EhCoactosin, an actin-binding protein of the ADF/cofilin family, participates in actin dynamics, and here we report our studies of this protein using both structural and functional approaches. According to in vitro binding assays, full-length EhCoactosin binds both F- and G-actin. Instead of acting to depolymerize or severe F-actin, EhCoactosin directly stabilizes the polymer. When EhCoactosin was visualized in E. histolytica cells using either confocal imaging or total internal reflectance microscopy, it was found to colocalize with F-actin at phagocytic cups.

EhCoactosin consists of a central core of β-sheets surrounded by α-helices. The central core is made up of five strands: β1(26–32), β2(37–44), β3(60–69), and β4(76–85) forming antiparallel strands while β5-strand (113–117) forms parallel strand with β3 and β4. The central β-sheets are flanked on both sides by a total of five helices; α1(9–17) and α3(92–107) are located on the N-terminal side, and α2(48–54), α4(120–122) and α5(125–137) are located on the C-terminal side. This arrangement of secondary structural elements is a common structural feature of proteins belonging to the ADF/cofilin family. The loop connecting strands β3 and β4, which has a conserved lysine at position 75, is called the “F-loop” and it is expected to participate in stabilizing and binding to F-actin. As described in more detail below, the surface of EhCoactosin is highly negatively charged, and this F-loop is part of the negatively charged surface. The N-terminal end and the F-loop are at two opposite sides of the globular structure suggesting that EhCoactosin binds G-actin and F-actin in very different ways. Although there is a general similarity of the overall conformation of EhCoactosin with that of related proteins in other organisms, the surface charge distributions of EhCoactosin is markedly distinctive. The overall structure of EhCoactosin is quite similar to that of human coactosin-like protein (HCLP), with an RMSD of 1.56 Å and few major differences. The N-terminal regions of the two proteins do deviate by up to 14.7 Å, with that of HCLP bent towards the inside of the structure while in EhCoactosin this N-terminal region is extended.

> MSGFDLSEVAGPVAEVIDDKNEEVEFVVFGVQTQPNKLVVDAKGKGGLEEVKAALKEDALQFAYYRTISGDEESKRVKFVFISWAGEGIKKPKLRAVMSILKGDVKNVINNFHIELHATSLDDLVEDEIAAKIKLEHHAHHH>[2x]MSSCKDSLSLMAMWGSIARFDPKHERSFEGPEKRLEVIMRVVDGTHVSGLLAHDDDVWQKVIDAICAHIVSREFNEYIRSYVLSE;>[2x]XSLFVMKDRVILITCGTITLLNCVPLICEAVSTVCGEVEWVSFMHKNYSFPWEQKGPHLSMAEEFKTLRSHFPSGQPFIFGPIDSDHYFLYFHSDVVQPSCSDDAQLSMTMYGLDRNQTKHWYSDKMLPTGPETAVIREATGLSEVVDDSWILHDLQYEPCGYSINAIRGSEYQTIHITPEEHCSFASYETNTCALNYSKCICGVLRVFDPERFSVIV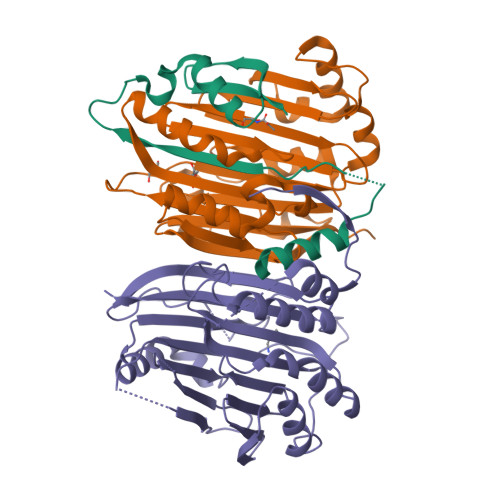FIDPDSAVGKSYHSGGTIGVEPEYYPNYEAHHRTVNEYTPGHWVLKVNYVKRAVGTVGTSAASGAKE;>[2x]MSVTRINQQTECPSSVHDLVSCWGGCTQSKTSTDSGLEKRFELNFAQPVDIGTVTVKQLASVMERAGESLRQNSAELGIHTLKFDRSLLVFTAKQIVVRSSVSVMLHEAVHPMLELMRSHNIIVDWASFMRVNYGSPWDMTSETSDIMAHEYAELKSAFPTGHPYLAGPVDRDHCFYFVYDGIDRDPSSCRRENDVQINVYMYNVQADDEYDLDGNTKEQQLLVSHCAGEYETLRVSTYGSTHPFASFETNAVSAASDITKIVNGLLKKFYPERVLLVLLQDRDAQGTTACGVMDRLEGFTVVHRGANHFGGGYVFHQATYARSA>GHHHHHHHHHHGLVPRGSHMYFQKARLIHAELPLLAPFKTSYGELKSKDFYIIELINEEGIHGYGELEAFPLPDYTEETLSSAILIIKEQLLPLLAQRKIRKPEEIQELFSWIQGNEMAKAAVELAVWDAFAKMEKRSLAKMIGATKESIKVGVSIGLQQNVETLLQLVNQYVDQGYERVKLKIAPNKDIQFVEAVRKSFPKLSLMADANSAYNREDFLLLKELDQYDLEMIEQPFGTKDFVDHAWLQKQLKTRICLDENIRSVKDVEQAHSIGSCRAINLKLARVGGMSSALKIAEYCALNE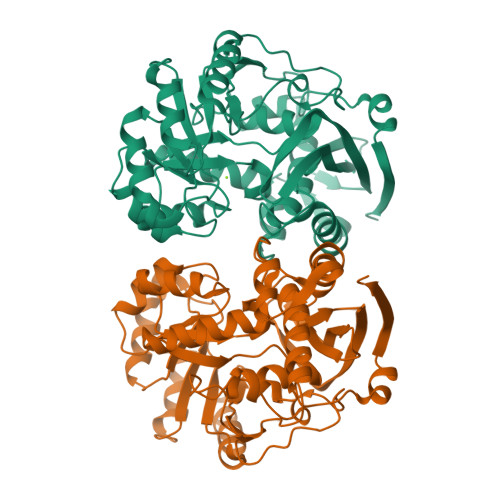ILVWCGGMLEAGVGRAHNIALAARNEFVFPGDISASNRFFAEDIVTPAFELNQGRLKVPTNEGIGVTLDLKVLKKYTKSTEEILLNKGWS[2x]>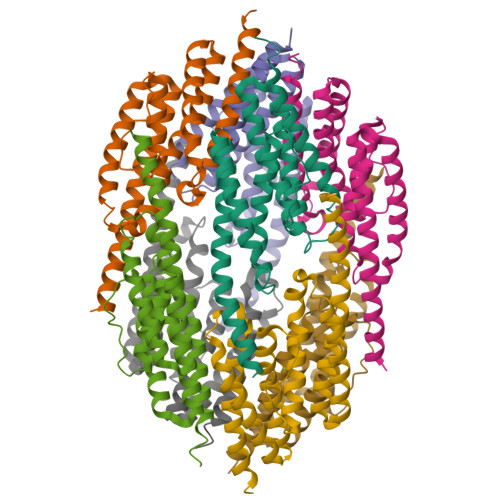GPHMRLEECRKRLEELEAAREELLKVLREMRIHSTKSIALIHAGKVEEAEQELKKAIELLEKVKAYREYPEIYFYLCNDAMQELVEAIAFKNAISGEFTFEIDLEVTPAAFLNGFADAVGELRRYALTKLIEGDFKSAERMLEVMEKIYERLMEFTTFPDKLVSGLRKKLDVARGGIERTKSDYIAAKVARLNESLGGN[8x]4-nitro-cinnamaldehyde | C9 H9 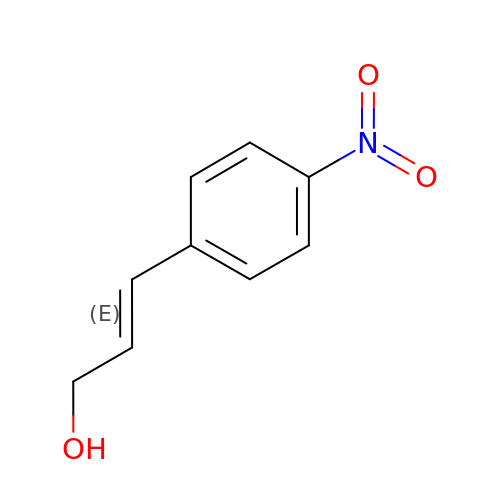N O3 | LGXXEDSIJZHDBN-OWOJBTEDSA-N> MLESKLKAPVFTATTQGDHYGEFVLEPLERGFGVTLGNPLRRILLSSIPGTAVTSVYIEDVLHEFSTIPGVKEDVVEIILNLKELVVRFLDPKMASTTLILRAEGPKEVRAGDFTPSADVEIMNPDLHIATLEEGGKLYMEVRVDRGVGYVPAERHGIKDRINAIPVDAIFSPVRRVAFQVEDTRLGQRTDLDKLTLRIWTDGSVTPLEALNQAVAILKEHLNYFANPEASLLPTPEVSKGEKRESAEEDLDLPLEELGLSTRVLHSLKEEGIESVRALLALNLKDLRNIPGIGERSLEEIRQALAKKGFT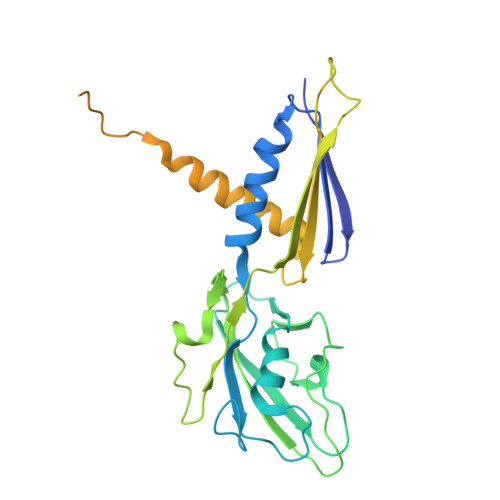LKE2-(butylsulfanyl)adenosine | C14 H21 N5 O4 S | 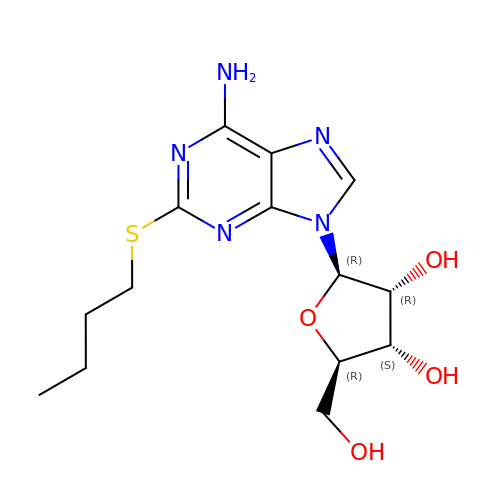JUZWTKSKLZRPBL-QYVSTXNMSA-N>[8x]MRVENNNVSGQNHDPEQIDLIDLLVQLWRGKMTIIISVIVAIALAIGYLAVAKEKWTSTAIITQPDVGQIAGYNNAMNVIYGQAAPKVSDLQETLIGRFSSAFSALAETLDNQEEREKLTIEPSVKNQQLPLTVSYVGQTAEGAQMKLAQYIQQVDDKVNQELEKDLKDNIALGRKNLQDSLRTQEVVAQEQKDLRIRQIQEALQYANQAQVTKPQIQQTGEDITQDTLFLLGSEALESMIKHEATRPLVFSPNYYQTRQNLLDIESLKVDDLDIHAYRYVMKPMLPIRRDSPKKAITLILAVLLGGMVGAGIVLGRNALRNYNAKEFRVPGSHHHHHHHH

Polysaccharide co-polymerases are a large family of membrane proteins that play an essential role in regulating the length distribution of the synthesized polysaccharide chain by interacting with the membrane-bound polymerase Wzy as it assembles the growing Oag or ECA polysaccharide of the LPS. Key to the Wzy-dependent pathway is the polysaccharide co-polymerase Wzz that is known to homo-oligomerize into a unique bell-shaped structure. As well as being assembled into bell-shaped structures common features include a membrane topology consisting of an N (TM1) and C (TM2) terminal transmembrane helix, an elongated periplasmic α-helical domain containing a predicted coiled-coil region and conserved sequence motifs such as a Proline-rich segment proximal to TM2 and a glycine-rich segment within TM2. With that in mind, we determined and herby report the structure of a fully intact example polysaccharide co-polymerase, WzzB, from E. coli by cryo-electron microscopy to an overall resolution of 3.0 Å.

Since an octameric complex is clearly visible in the unsymmetrized map, 8-fold (C8) symmetry was applied which led to a marked improvement in overall resolution to 3.0 Å. The high quality of the map allowed ~95% of the amino acid sequence to be unambiguously built, revealing structural details of the transmembrane and cytoplasmic domains as well as a highly conserved proline-rich segment proximal to the C-terminal transmembrane helix. Herein, the loop is positioned on the inside of the cavity and extends to the center of the periplasmic domain in a similar conformation as seen in the structure of a Salmonella typhimurium/Shigella flexneri WzzB chimera. While the first two prolines of this motif are seen in the trans conformation, P293 is best modeled in the cis-conformation in the density of our structure. The cis-conformation of the ω torsion angle of proline 293 creates a unique kink in this linker region thus helping to direct the C-terminal transmembrane helix into position. In the octameric assembly, the 2-helix bundles are ~32 Å apart (when measured from center to center) and do not interact with one another. Within each bundle their closest interactions are at their cross-point, which perhaps not surprisingly, coincides with the conserved GXXXG motif that has been found in ~50% of all α-helical membrane proteins and is suggested to be involved in helix-helix packing. Each of the pillars is tilted slightly inward toward the center of the chamber, reducing the inner diameter from ~75 Å on the periplasmic side to ~64 Å on the cytoplasmic side and the outer diameter from ~100 Å on the periplasmic side to ~83 Å on the cytoplasmic side. However, at the N-terminal end of the protein, a short amphipathic helix (α0) runs parallel to the membrane and interacts with TM2 of its helix bundle as well as with TM2 of the neighboring protomer, which curves slightly toward α0.>GMAVSSNGGAIKAVIYDCDGVMFDSFEANLAFYQRIMEMMGRPRLSRDNEEQMRILHTYANREVLAHFFPSPGDWEEAVRCAGAIDYRELVPLMIMEEGFREALDTLKGRVGLGVCTNRSTS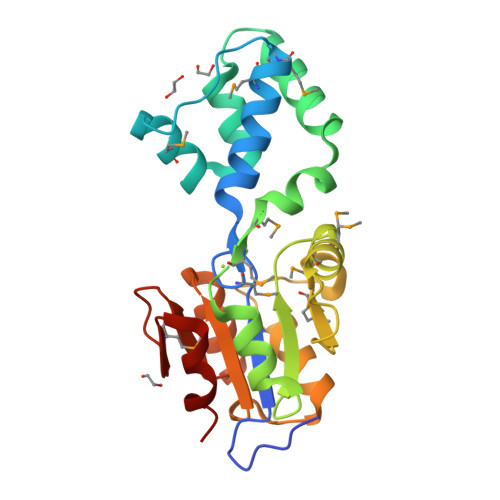MDMVLRLFSLDSYFSIVMTASRVTNPKPHPEPLLKVLEHFGIGPREALFVGDSEVDRLSAEAAGVPFVAYKAPLPAAYRMEHHREIIDLLG[2x]>AECSVDIQGNDQMQFNTNAITVDKSCKQFTVNLSHPGNLPKNVMGHNFVLSTAADMQGVVTDGMASGLDKDFLKPDDSRVIAQTKLIGSGEKDSVTFDVSK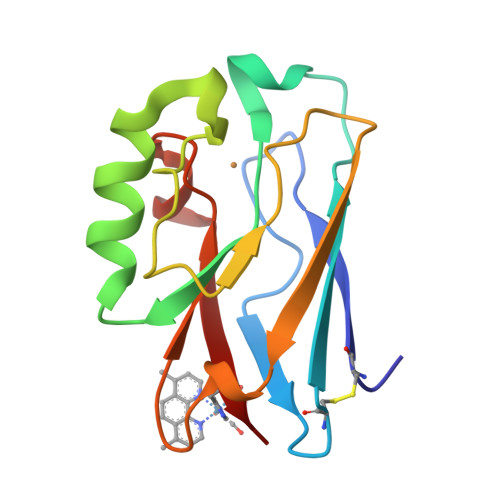LKEGEQFMFFCTFPGHSALMWGFLHLK[4x]5-[2-(4-methylphenyl)sulfanylethanoyl]-1,3-dihydroindol-2-one | C17 H15 N 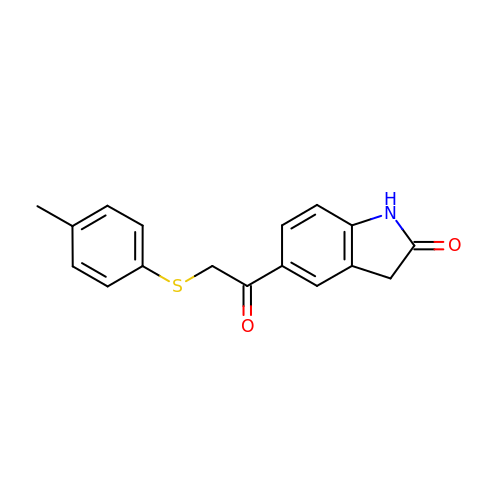O2 S | RXONTIZYFOQKAA-UHFFFAOYSA-N>[6x]MTTTRQDTQWQQLTEHWQELADFGGIEALLGWDQSTFLPAGAAEDRARQQSLLAGLRHARATDAGYGKLLDAASSRSDLSPEQARMVQVARQDFEKATRIPAEFVREFSGHVGQSYSAWTEARPANDFGRMVPYLEKTLDLSLQAASYFPEFGDPLDYYINESDEGMTA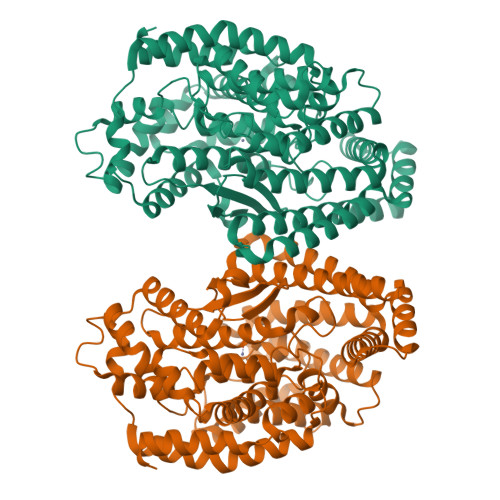EQVGQVFAELRAALVPLADAVIAAGAPRTDFLGRGFAQERQLAFGERVIRDYGYDFRRGRQDLTHHPFMTRLGGHDVRITTRVKEQDPTDALYSTLHEAGHALYEQGVDAAFLGTPLGGGVSAGVHESQSRLWENLVGRSRAFWAAYFGDWRDTFPEQLAGVTEEEMYRAVNTVSRSLIRTDADELTYNLHVITRFELEREMLAGKLAVRDLADAWHAAYEQNLGLRAPSDVDGALQDVHWYFGPIGGSFQGYTIGNVLSAQFYAAAEAANPGLEADFARKDFSRLHGWLRENVYRHGRRWTPGELIERATGQALTAGPYLKYLRGKYGELYGV>MERKISRIHLVSEPSITHFLQVSWEKTLESGFVITLTDGHSAWTGTVSESEISQEADDMAMEKGKYVGELRKALLSGAGPADVYTFNFSKESAYFFFEKNLKDVSFRLGSFNLEKVENPAEVIRELIAYALDTIAENQAKNEHLQKENERLLRDWNDVQGRFEKAVSAKEALETDLYKRFILVLNEKKTKIRSLHNKLLNAAQEREKDIKQEG[2x];> PSTKEHFAREYDCYGDS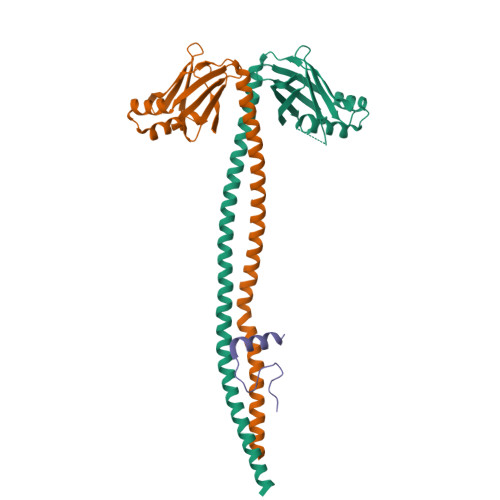YFIDTDLNQLKEVFSGIKNS>SLVELGKMILQETGKNPVTSYGAYGCNCGVLGRGKPKDATDRCCYVHKCCYKKLTDCNPKKDRYSYSWKNKTIVCGENNACLKELCECDKAVAICLRENLDTYNKKYKNNYLKPFCDK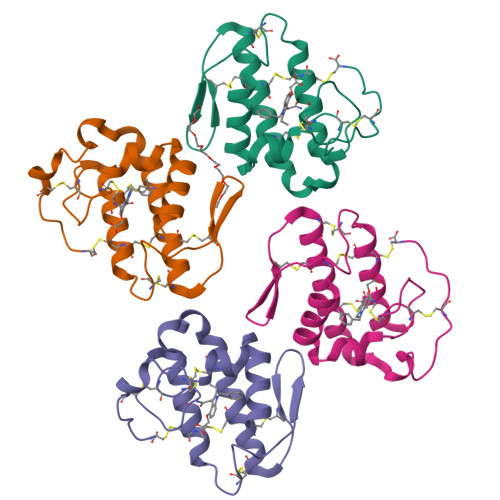ALPC[4x]> IVGGYKCEKNSQPWQVAVINEYLCGGVLIDPSWVITAAHCYSNNYQVLLGRNNLFKDEPFAQRRLVRQSFRHPDYIPLIVTNDTEQPV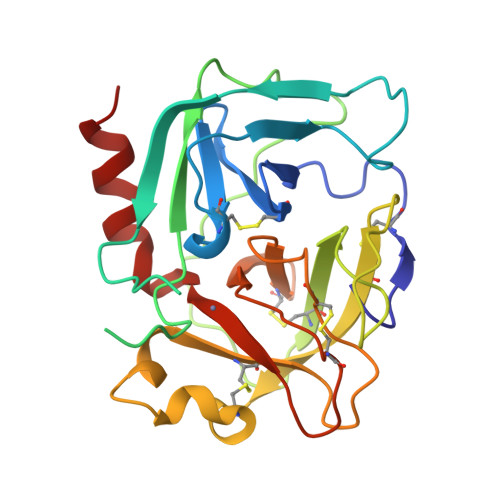HDHSNDLMLLHLSEPADITGGVKVIDLPTKEPKVGSTCLASGWGSTNPSEMVVSHDLQCVNIHLLSNEKCIETYKDNVTDVMLCAGEMEGGKDTCAGDSGGPLICDGVLQGITSGGATPCAKPKTPAIYAKLIKFTSWIKKVMKENP>MWFGEFGGQYVPETLIGPLKELEKAYKRFKDDEEFNRQLNYYLKTWAGRPTPLYYAKRLTEKIGGAKVYLKREDLVHGGAHKTNNAIGQALLAKFMGKTRLIAETGAGQHGVATAMAGALLGMKVDIYMGAEDVERQKMNVFRMKLLGANVIPVNSGSR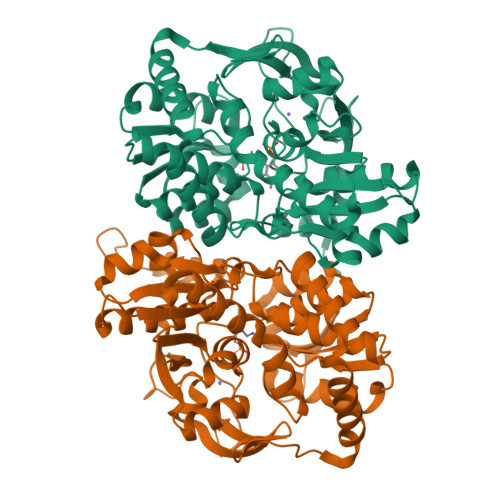TLKDAINEALRDWVATFEYTHYLIGSVVGPHPYPTIVRDFQSVIGREAKAQILEAEGQLPDVIVACVGGGSNAMGIFYPFVNDKKVKLVGVEAGGKGLESGKHSASLNAGQVGVSHGMLSYFLQDEEGQIKPSHSIAPGLDYPGVGPEHAYLKKIQRAEYVAVTDEEALKAFHELSRTEGIIPALESAHAVAYAMKLAKEMSRDEIIIVNLSGRGDKDLDIVLKVSGNVLEHHHHHH[4x]> PVV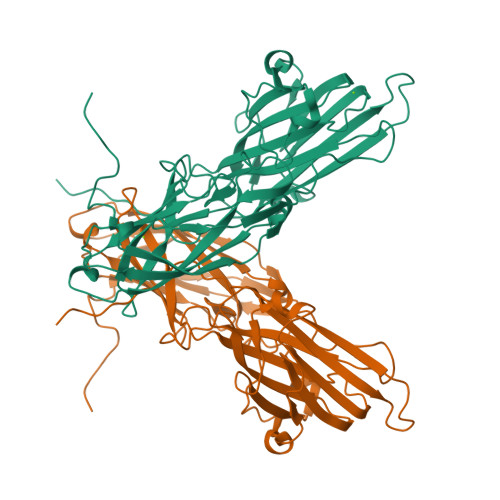NVADAKGTNVNDKVTASNFKLEKTTFDPNQSGNTFMAANFTVTDKVKSGDYFTAKLPDSLTGNGDVDYSNSNNTMPIADIKSTNGDVVAKATYDILTKTYTFVFTDYVNNKENINGQFSLPLFTDRAKAPKSGTYDANINIADEMFNNKITYNYSSPIAGIDKPNGANISSQIIGVDTASGQNTYKQTVFVNPKQRVLGNTWVYIKGYQDKIEESSGKVSATDTKLRIFEVNDTSKLSESYYADPNDSNLKEVTDQFKNRIYYEHPNVASIKFGDITKTYVVLVEGHYDNTGKNLKTQVIQENVDPVTNRDYSIFGWNNENVVRYGGGSADGDSAV>[2x]HHHHHHMNKVLLLSIQNPLYPITVDVLYTVCNPVGKVQRIVIFKRNGIQAMVE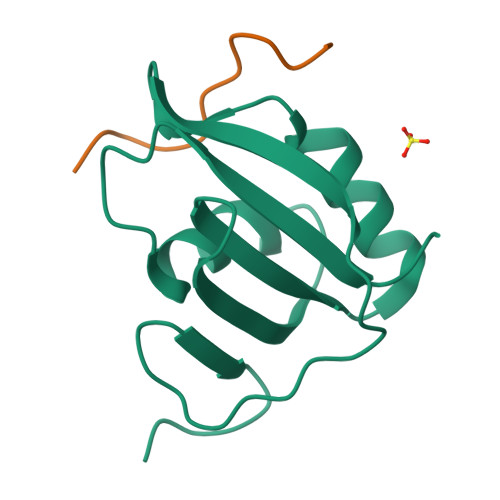FESVLCAQKAKAALNGADIYAGCCTLKIEYARPTRLNVIRNDNDSWDYTKPYLGRRD;>SNPNAGKVLLPTP[2x]> GSMEDDAETKAKAEDLK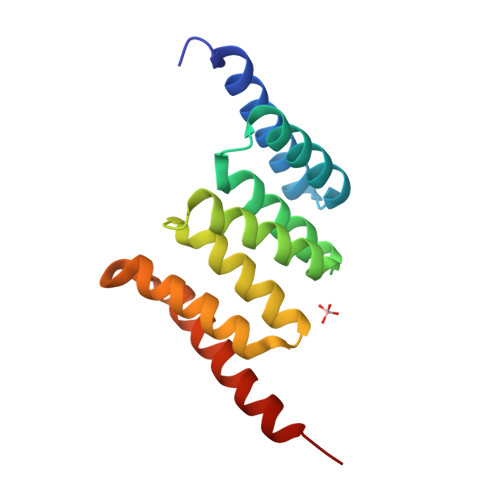MQGNKAMANKDYELAINKYTEAIKVLPTNAIYYANRAAAHSSLKEYDQAVKDAESAISIDPSYFRGYSRLGFAKYAQGKPEEALEAYKKVLDIEGDNATEAMKRDYESAKKKVEQSLNLEKTV> GCGGAUUUAGCUCAGUUGGGAGAGCGCCAGACUGAAG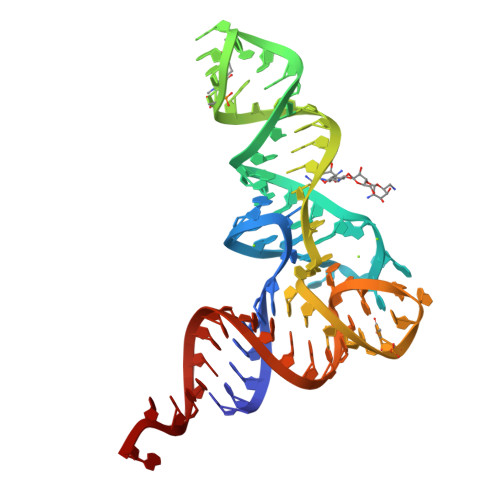AUCUGGAGGUCCUGUGUUCGAUCCACAGAAUUCGCACCA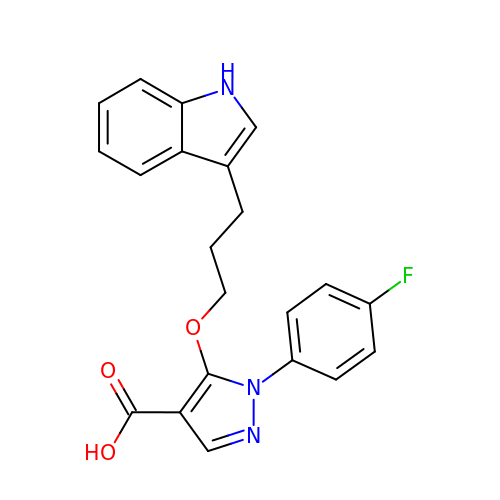1-(4-fluorophenyl)-5-[3-(1H-indol-3-yl)propoxy]-1H-pyrazole-4-carboxylic acid | C21 H18 F N3 O3 | HECYVAQVQUQMCB-UHFFFAOYSA-N> DYTVHDTDGKPVLNN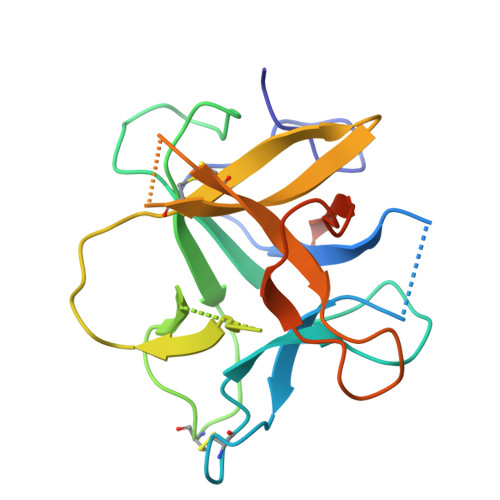AGQYYILPAKQGKGGGLGLSNDDDGNCPLTVSQTPIDIPIGLPVRFSSRARISHITTALSLNIEFTIAPACAPKPARWRIFDEQSSEKGYTPVKISDDFSSAAPFQIKKFEEDYKLVYCSKSESGERKCVDLGIKIDNEKNRRLVLKEGDPFKVKFKKVDEESSEEWSIV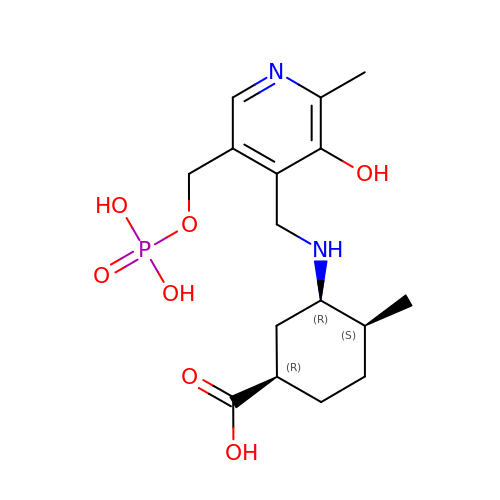(3~{S},4~{S})-4-methyl-3-[[2-methyl-3-oxidanyl-5-(phosphonooxymethyl)pyridin-4-yl]methylamino]cyclohexene-1-carboxylic acid | C16 H25 N2 O7 P | VMGXIUNFRDERKW-FGBBXPCBSA-N> MDPEFMSSVDVLLTVGKLDASLALLTTQDHHVIEFPTVLLPENVKAG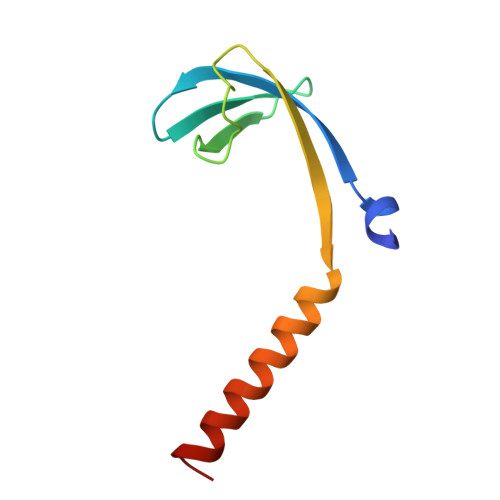SIIKMQVSQNLEEEKKQRNHFKSIQAKILEKYGTH>GAMAQELKERAKVFAKPIGASYQGILDQLDLVHQAKGRDQIAASFELNKKINDYIAEHPTSGRNQALTQLKEQVTSALFIGKMQVAQAGIDAIAQTRPELAARIFMVAIEEANGKHVGLTDMMVRWANEDPYLAPKHGYKGETPSDLGFDAKYHVDLGEHYADFKQWLETSQSNGLLSKATLDESTKTVHLGYSYQELQDLTGAESVQMAFYFLKEAAKKADPISGDSAEMILLKKFADQSYLSQLDSDRMDQIEGIYRSSHETDIDAWDRRYSGTGYDELTNKLASATGVDEQLAVLLDDRKGLLIGEVHGSDVN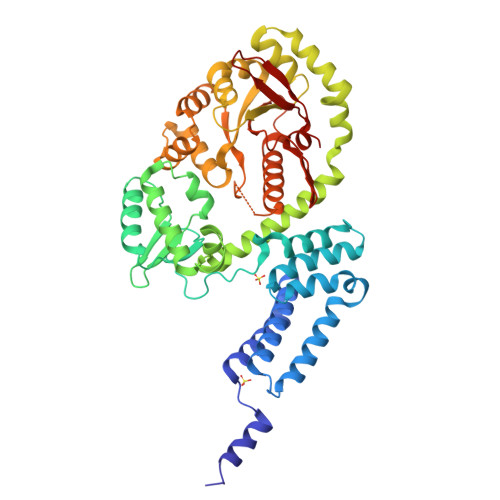GLRFVNEQMDALKKQGVTVIGLEHLRSDLAQPLIDRYLATGVMSSELSAMLKTKHLDVTLFENARANGMRIVALDANSSARPNVQGTEHGLMYRAGAANNIAVEVLQNLPDGEKFVAIYGKAHLQSHKGIEGFVPGITHRLDLPALKVSDSNQFTVEQDDVS[4x]>GPGRAPPSPDLRADEPKTPCLVGGAHAFILKISSFCGLAPLRFEPRSQEYAVTISKGKCFYSYILVTFLVICTIYGLVAEIGVGVEKSVRMSSRMSQVVSACDILVVAVTAGVGVYGAPARMRTMLSYMENIVAVDRELGRHHSAATERKLCALLLLILLSFTILLVDDFCFYAMQAGKTGRQWEIVTNYAGFYFLWYIVMVLELQFAFTALSLRARLKLFNEALNVTASQVCKPVKKPKNSQLSVYATSVRPVSCKRENVIVETIRVRDKDDAFVMMKTADGVPCLQVPPCEAVGRLSRMRCTLCEVTRHIADGYGLPLVIILMSTLLHLIVTPYFLIMEIIVSTHRLHFLVLQFLWCTTHLIRMLVVVEPCHYTIREGKRTEDILCRLMTLAPHGGVLSSRLEVLSRLLMLQNISYSPLGMCTLDRPLMVTVLGAVTTYLVILIQF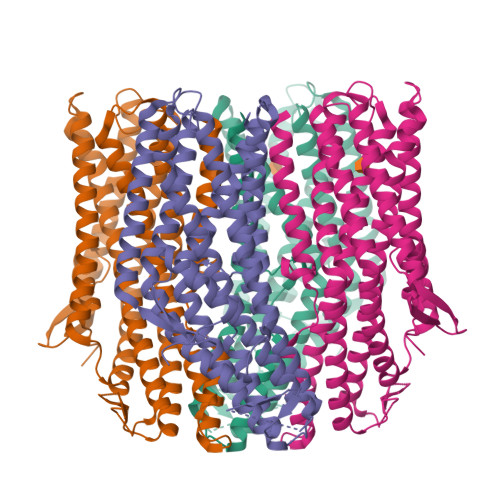QRYDS[4x]> GPLGSMEGAPDINIILENSLSPDATLRHAAEQQLTHAAETNFSQYLLTLVQALANESSEGHIRAAAGIALKNAFSAREFARQAALQAKWLNQTDQETRTRVKQLALETLASSNSKAGQAAAQVIAAIAAIELPRNQWPELMHALVRNVSEGGQHQKQASLTAIGFICETQDTDLRNSLVGHSNAILTAVVQGARKEEPNNEVRFAAITALGDSLEFVGNNFKHEGERNYIMQVVCEATQAQDSRIQQGAFGCLNRIMALYYEHMRYYMEKALFGLTILGMKSDDEDVAKLAVEFWSTVCEEEIAIEDDNAQVESSEQMRPFYNFARVATNEVVPVLLQLLTKQDEDASDDEYNISRAAYQCLQLYAQAVGSTIIPPVIQFVEHNLRHADWHFRDAAVSAFGAIMDGPEEKVLEPIVKTGMQPLIAMMEDESIQVRDSTAYALGRITEACSEAIDPNTHLEPLIRSLFNGLMNSPKMAASCCWALMNIAERFAGEPGAAQNPLTPHFNQSVTNLLTVTA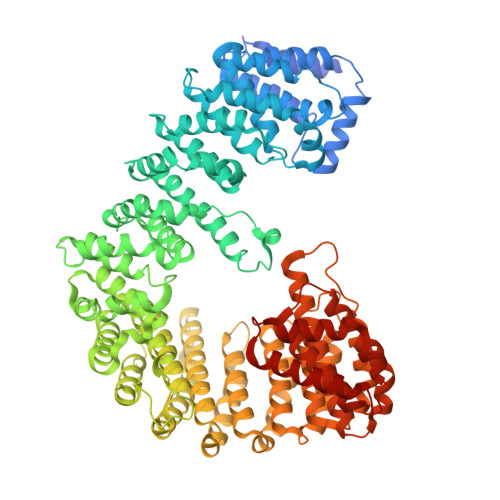PMNGDSTVRTAAYEVLSVFVQNAANDSLSAVASLSTVILQRLEETLPLQQQVVSVEDKLILEDMQTSLCTVLQATVQRLDKEIAPQGDRIMQVLLQILSTCGGKSSVPEGVFAAISALANAMEEEFAKYMEAFAPFLYNALGNQEEPSLCSMAIGLVSDVTRSLGERSQPYCDNFMNYLLGNLRSTTLANQFKPAILQCFGDIASAIGGHFETYLTIVAQVLQQAATITAGPDGSYEMIDYVISLREGIMDAWGGIIGAMKTSNKTNVLQPYVESIFALLNSIANDPNRSEALMRASMGVIGDLADAYPNGQLADAFRQDWITAMIRETRSNREFGARTIETARWAREQVKRQIAGSQTVMQQS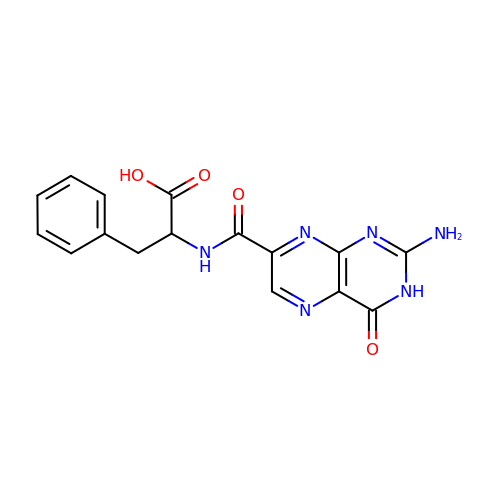(2R)-2-[(2-azanyl-4-oxidanylidene-3H-pteridin-7-yl)carbonylamino]-3-phenyl-propanoic acid | C16 H14 N6 O4 | AJHMFJMLQDPCOX-UHFFFAOYSA-N>[4x]MKILKLQTLRGPNYWSIHRHKLVVMRLDLEDLYEKYTSDIPGFYKGLTEVLPSLVEHLCSPGVKGGFLTRVEKGTLIGHVIEHVAIELQELAGMPVGFGRTRETSTTGVFQVVIEYENEQAGRYAARAAVRLCQSIVDTGTYPATELQQD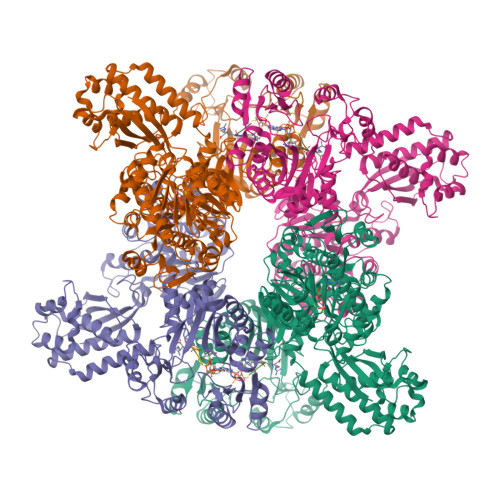LEDLKELKNQASLGPSTEAIVKEAEARGIPWTQLGARFMIQFGYGVNQKKIQATLSNQTGILGVELACDKEGTKRILKDAGVPVPRGTVARYFDELQDAIEYVGGYPIVIKPLDGNHGRGITIDVKNWQEAEEAYDLARKASKTKTVIVERYYTGKDHRVLVVNGKVVAVAERVPAHVVGNGKSTIAELIEETNRDPQRGDGHDNILTRITVDKSALDILGKQGYSIDSIPLKGKKCFLRATANLSTGGIAVDRTDEIHPENVWLLSRVAKIIGLDIAGIDVVTEDISQPLREVEGVIVEVNAAPGFRMHVAPSRGLARNVAGAVMDMLFPGSKNGRIPILSVTGTNGKTTTTRLLAHIIKQTGKVVGYTTTDGTYIGEYLAETGDNTGPQSAHLILSDPTVEVAVLETARGGILRSGLGFSSCEVGIVLNVTADHLGIGDIDTIEQLAKLKSVVAESVMPKGYAVLNAEDPLVAAMADRVKGQVAYFSMDPNNELLLRHTEAGGLAAIYENGYISILKGDWTLRIEKAVNVPITMAGKAPFMIANALAACLAVFTQGVKIEHIRKGLSTFVASVDQTPGRMNMFNMGSYHALVDYAHNPASYEALGGFVRNWPGKRIGVVGGPGDRRDEDFVSLGELAADIFDEIIIKEDDDTRGRPRGNAAELICQGVKQFLNGIKNSESKATYESILDETAAINTALDRAPIDGLVVILPESVNRAISLIEGRHVIQDIELLQDSQREPKDQEVLKSSILEHHHHHH;>DDDD[4x]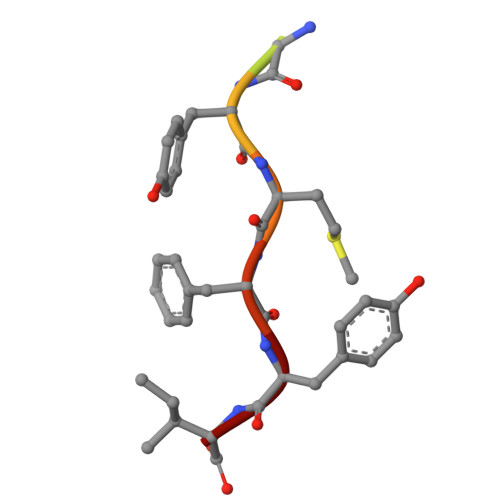> EDLDGYMFYI> ASSPTPPRGVTVVNNFDAKRYLGTWYEIARFDHRFERGLEKVTATYSLRDDGGLNVINKGYNPDRGMWQQSEGKAYFTGAPTRAALKVSFFGPFYGGYNVIALDREYRHALVSGPDRDYLWILSRTPTISDEVKQEMLAVAT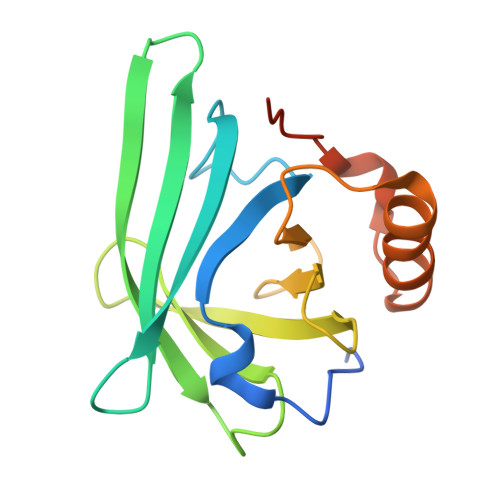REGFDVSKFIWVQQPGSAWSHPQFEK> GSHMKNSVSVDLPGSMKVLVSKSSNADGKYDLIATVDALELSGTSDKNNGSGVLEGVKADASKVKLTISD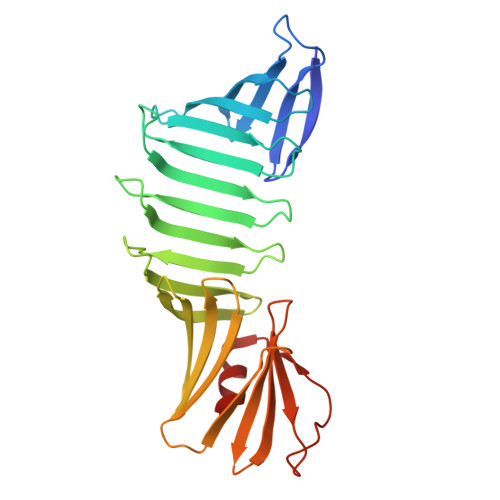DLGQTTLEVFKSDGSTLVSKKVTSKDKSSTEEKFNEKGEVSEKIITRADGTRLEYTGIKSDGSGKAKEVLKGYVLEGTLTAEKTTLVVKEGTVTLSKNISKSGAVSVELNDTDTKKTAAWNSGTSTLTITVNSKKTKDLVFTSSNTITVQQYDSNGTSLEGSAVEITKLDEIKNALK>MRGSHHHHHTTGEDDESECVINYVEKAVNKLTLQMPYQLFIGGEFVDAEGSKTYNTINPTDGSVICQVSLAQVSDVDKAVAAAKEAFENGLWGKINARDRGRLLYRLADVMEQHQEELATIEALDAGAVYTLALKTHVGMSIQTFRYFAGWCDKIQGATIPINQARPNRNLTLTKKEPVGVCGIVIPWNYPLMMLSWKTAACLAAGNTVVIKPAQVTPLTALKFAELTLKAGIPKGVVNILPGSGSLVGQRLSDHPDVRKIGFTGSTEVGKHIMKSCALSNVKKVSLQLGGKSPLIIFADCDLNKAVQMGMSSVFFNKGENCIAAGRLFVEESIHNQFVQKVVEEVEKMKIGNPLERDTNHGPQNHEAHLRKLVEYCQ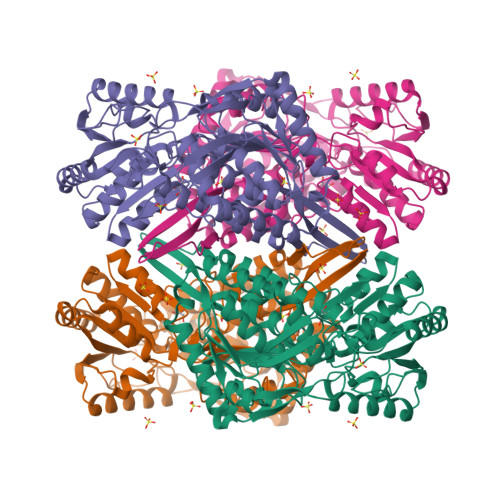RGVKEGATLVCGGNQVPRPGFFFQPTVFTDVEDHMYIAKEESFGPIMIISRFADGDVDAVLSRANATEFGLASGVFTRDINKALYVSDKLQAGTVFINTYNKTDVAAPFGGFKQSGFGKDLGEAALNEYLRIKTVTFEY[4x]>[24x]SVDTMALWLGLRAVLVVAGLAVLLQLIRGWLSSKSYVF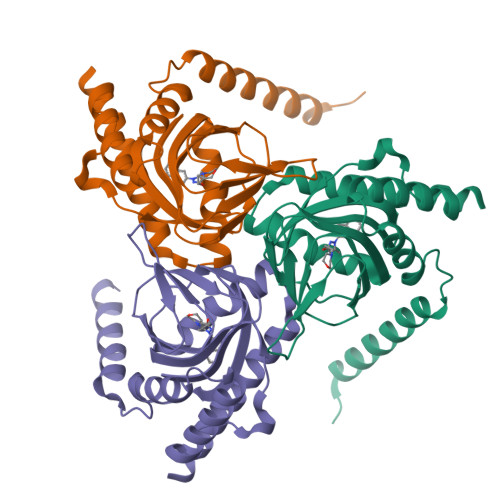NREEIARLAKEHSGLDYEVAFSKIIVELRKKHPGHILQDEDLQWVFVNAGGWMGSMCLLHASLTEYVLLFGTAVDTGGHSGRYWAEISDTILSGTFRQWKEGTTKSEIFYPGDTIVHEVGEATSVQWSSGTWMVEYGRGFIPSTCAFALADTIFSTQDFLTLFYTVKVCSKALLLEASTHLSQLGFF> GSAKDPHNHYIWAKLSAYHIAELLEQEKRYDESLAIIEEARVIWPNVPEFPLKKANILYVNHQLEDAKEIYQSLLENAAIDYQP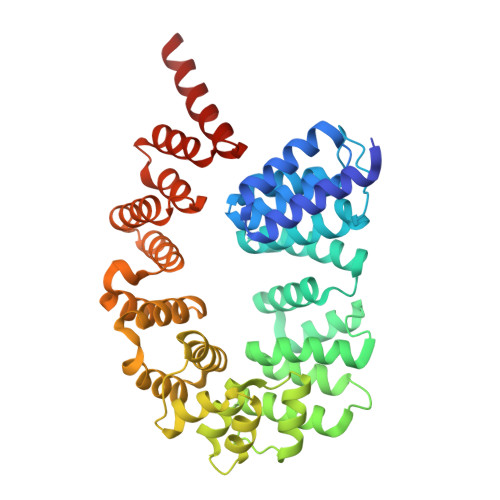IVLYEATNFMPHKMLGTIYLEEKDYTRAMTHFSKAYAENSSDYGVMFQMIMLLSKFHQPKEIFAFMERHHFISSTETGLRLLSMTTQQGYAELSELIVQSLTDVYPPVAEATEVKIATIRNVFPVISESAILFGIKEELIDAADLCLWHYENPQLPIENVMKNSDVGDIYDFIFENGPRISKKRYLFVLERAIALGKGEFADYLLALRNVYHDSINSHIADLFFQYDFADIALDFYNIVDADEVTKQGYINLINYLVDADVLDEALAIAERGIDNFSTDFRFYLWAIKIDTENRANRISEAMDEFPNNRYLAKLLDEVTMLQDTVTNNR>MNKNNTKLSTRALPSFIDYFNGIYGFATGIKDIMNMIFKTDTGGDLTLDEILKNQQLLNDISGKLDGVNGSLNDLIAQGNLNTELSKEILKIANEQNQVLNDVNNKLDAINTMLRVYLPKLTSMLSDVMKQNYALSLQIEYLSKQLQEISDKLDIINVNVLINSTLTEITPAYQRIKYVNEKFEELTFATETSSKVKKDGSPADILDELTELTELAKSVTKNDVDGFEFYLNTFHDVMVGNNLFGRSALKTASELITKENVKTSGSEVGNVYNFLIVLTALQAKAFLTLTTCRKLLGLADIDYTSIMNEHLNKEKEEFRVNILPTLSNTFSNPNYAKVKGSDEDAKMIVEAKPGHALIGFEISNDSITVLKVYEAKLKQNYQVDKDSLSEVIYGDMDKLLCPDQSEQIYYTNNIVFPNEYVITKIDFTKKMKTLRYEVTANFYDSSTGEIDLNKKKVESSEAEYRTLSANDDGVYMPLGVISETFLTPINGFGLQADENSRLITLTCKSYLRELLLATDLSNKETKLIVPPSGFISNIVENGSIEEDNLEPWKANNKNAYVDHTGGVNGTKALYVHKDGGISQFIGDKLKPKTEYVIQYTVKGKPSIHLKDENTGYIHYEDTNNNLEDYQTINKRFTTGTDLKGVYLILKSQNGDEAWGDNFIILEISPSEKLLSPELINTNNWTSTGSTNISGNTLTLYQGGRGILKQNLQLDSFSTYRVYFSVSGDA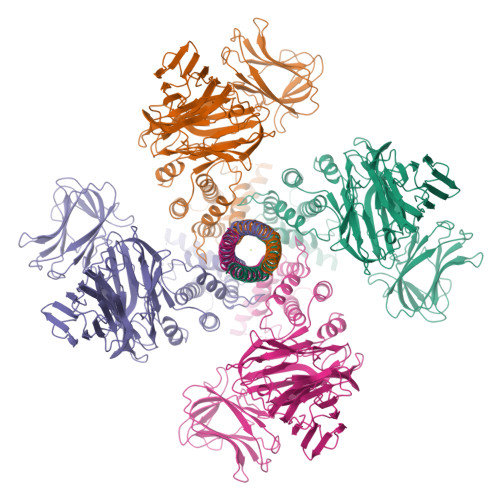NVRIRNSREVLFEKRYMSGAKDVSEMFTTKFEKDNFYIELSQGNNLYGGPIVHFYDVSIK[4x]>[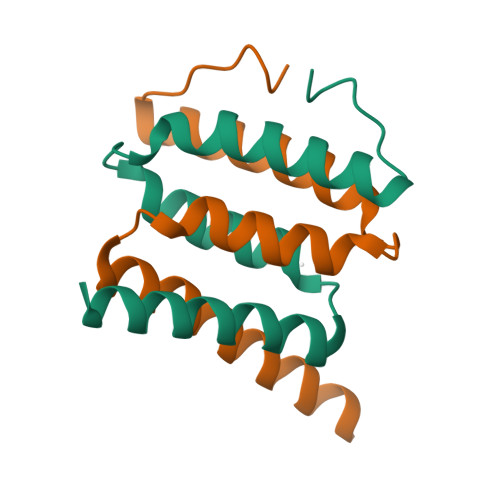4x]AVYGIDAMNPSSRDDFTEFGKLLKDKITQYEKSLYYASFLEVLVRDVCISLEIDDLKKITNSLTVLCSEKQKQEKQSKAK> MEGLAGYVYKAASEGKVLTLAALLLNRSESDIRYLLGYVSQQGGQRSTPLIIAARNGHAKVVRLLLEHYRVQTQQTGTVRFDGYVIDGATALWCAAGAGHFEVVKLLVSHGANVNHTTVTNSTPLRAACFDGRLDIVKYLVENNANISIANKYDNTCLMIAAYKGHTDVVRYLLEQRADPNAKAHCGATALHFAAEAGHIDIVKELIKWRAAIVVNGHGMTPLKVAAESCKADVVELLLSHADCDRRSRIEALELLGASFANDRENYDIIKTYHYLYLAMLERFQDGDNILEKEVLPPIHAYGNRTECRNPQELESIRQDRDALHMEGLIVRERILGADNIDVSHPIIYRGAVYADNMEFEQCIKLWLHALHLRQKGNRNTHKDLLRFAQVFSQMIHLNETVKAPDIECVLRCSVLEIEQSMNRVKNISDADVHNAMDNYECNLYTFLYLVCISTKTQCSEEDQCKINKQIYNLIHLDPRTREGFTLLHLAVNSNTPVDDFHTNDVCSFPNALVTKLLLDCGAEVNAVDNEGNSALHIIVQYNRPISDFLTLHSIIISLVEAGAHTDMTNKQNKTPLDKSTTGVSEILLKTQMKMSLKCLAARAVRANDINYQDQIPRTLEEFVGFH;> RPRREALFFPSQVTCTEALLRAPGAELAELPEGCPCGLPHGESALSRLLRALLAARASLDLCLFAFSSPQLGRAVQLLHQRGVR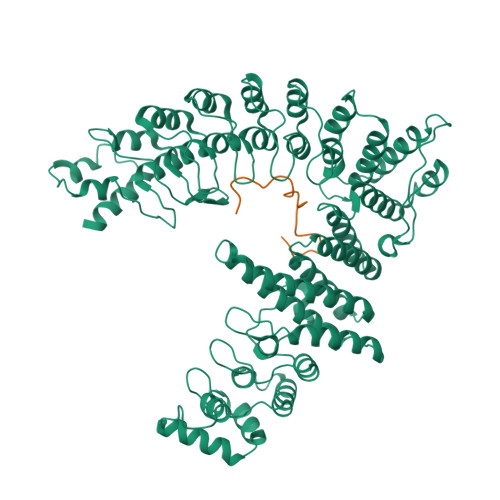VRVVTDCDYMALNGSQIGLLRKAGIQVRHDQDPGYMHHKFAIVDKRVLITGSLNWTTQAIQNNRENVLITEDDEYVRLFLEEFERIWEQFNPTKYTFFPPKKSHGSCAPPVSRAGGRLLS>MGRGKVKPNRKSTGDNSNVVTMIRAGSYPKVNPTPTWVRAIPFEVSVQSGIAFKVPVGSLFSANFRTDSFTSVTVMSVRAWTQLTPPVNEYSFVRLKPLFKTGDSTEEFEGRASNINTRASVGYRIPTNLRQNTVAADNVCEVRSNCRQVA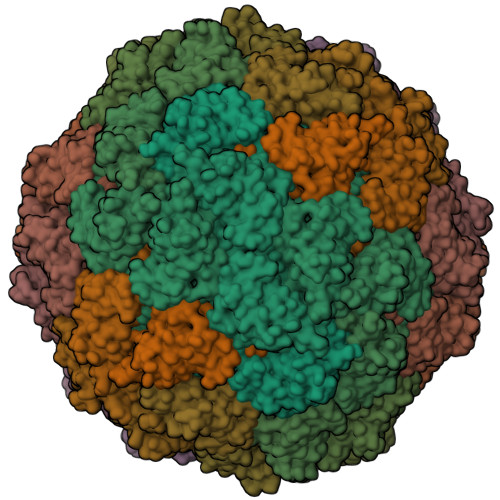LVISCCFN[30x]> MKAEGIKSPSAKYHDMAGSQRIPHKNPHIQKVAVLQSKPNKEDALNLIKEIAHKVSYLMKENH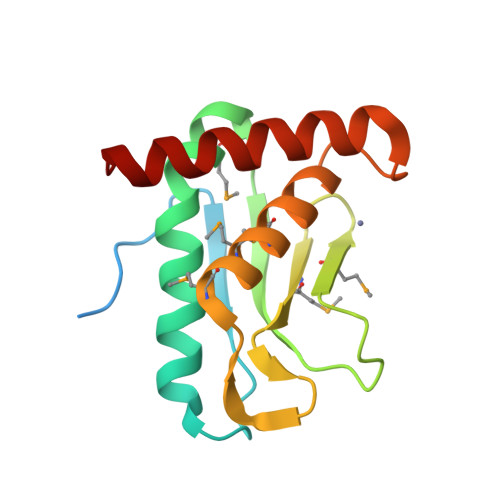FKVTNLVEFYPRDQRLLGMNVNHGSKIMLRLRCSTDEFQFLPMECIMGTMLHELTHNLFGPHDKKFYNKLDELIGRQWVIEQRGL~{N}-methyl-3-propan-2-yl-1~{H}-pyrazolo[3,4-c]pyridine-4-carboxamide | C11 H14 N4 O | 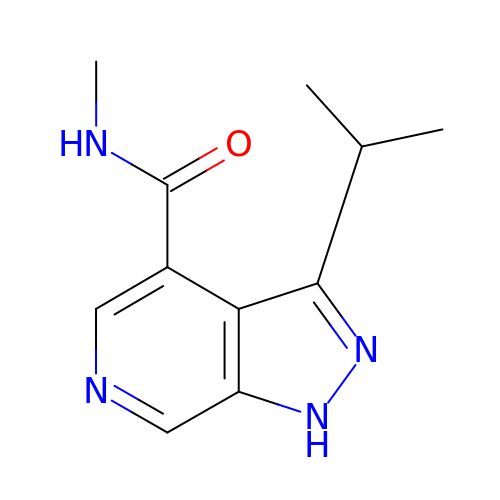GEGYOOMXCGLHBJ-UHFFFAOYSA-N>MSLRNDAYSTLRVSSEHGVARIILDNPPVNVIGATMMRELRT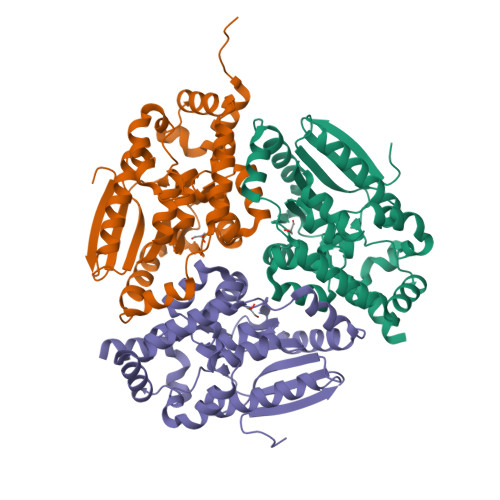VLTTLADDSSVRVIVFSSADPEFFLAHVDMRIGEKMDALQELAASAPADVNVFQAVGELIRHQPQVTIVKLAGKARGGGAEFVAAADMAFAAAETAGLGQIEALMGIIPGGGGTQYLRGRVGRNRALEVVLTADLFDAETAASYGWINRALPADELDEYVDRVARNIAALPDGVIEAAKRSLPADDLKEGLLGENDAWAATFSLPAAQQLISGGLKDGAQTPAGERDLEGLMRSVAREGHHHHHH[3x]>APAEILNGKEISAQIRARLKNQVTQLKEQVPGFTPRLAILQVGNRDDSNLYINVKLKAAEEIGIKATHIKLPRTTTESEVMKYITSLNEDSTVHGFLVQLPLDSENSINTEEVINAIAPEKDVDGLTSINAGRLARGDLNDCFIPCTPKGCLELIKETGVPIAGRHAVVVGRSKIVGAPMHDLLLWNNATVTTCHSKTAHLDEEVNKGDILVVATGQPEMVKGEWIKPGAIVIDCGINYVPDDKKPNGRKVVGDVAYDEAKERASFITPVPGGVGPMTVAMLMQSTVESAKRFLEKFKPGLEHHHHHH[4x]

Methylenetetrahydrofolate dehydrogenase/cyclohydrolase 2 (MTHFD2) is a bifunctional metabolic enzyme found in mitochondria, exhibiting both dehydrogenase and cyclohydrolase catalytic activities. In one-carbon metabolism, MTHFD2 converts 5, 10-methylene tetrahydrofolate (5,10-CH2-THF) to 10-formyl tetrahydrofolate (10-CHO-THF) in mitochondria, thereby regulating the production of NADH, purines, and pyrimidines. An isozyme, methylenetetrahydrofolate dehydrogenase, cyclohydrolase and formyltetrahydrofolate synthetase 1 (MTHFD1), performs similar catalytic reactions to MTHFD2, albeit localized in the cytoplasm rather than the mitochondrion. The key distinction between these two proteins lie in their expression profiles: MTHFD1 is typically expressed in normal cells while MTHFD2 is abundantly expressed in immortal, embryonic, and cancer cells, but absent in adult normal cells.

LY374571 was a competitive inhibitor of human MTHFD1 (IC50 = 630 nM) and MTHFD2 (IC50 = 80 nM). To investigate the molecular basis of the selectivity toward MTHFD2 over MTHFD1, cocrystal structures of human MTHFD1 were determined in complex with 16a, 16d, 16e, 16g, and LY374571 in the presence of NADP+, with resolutions ranging from 1.99 to 2.50 Å. Superimposition of the MTHFD1/16e complex structure with MTHFD1/LY374571 complex structure uncovered several differences between them. First, in the structure of MTHFD1/LY374571, the nicotinamide group of NADP+ was hydrogen bonded with the NH2 moiety of the triaminopyrimidine headgroup of LY374571. However, the addition of a chloride substituent on the phenyl ring in 16e induced a clash with the nicotinamide group of NADP+, leading to the shift of the nicotinamide group of NADP+ away from the triaminopyrimidine headgroup of 16e and the consequent loss of the hydrogen bond between 16e and NADP+ Instead, NADP+ in MTHFD1/16e structure was found to be hydrogen bonded with the side chain of Thr279. Second, in comparison with the MTHFD1/LY374571 structure, it was observed that the addition of the chloride atom in 16e led to the rotation of the phenyl ring by approximately 26°, accompanied by the movement of the γ-carboxylic acid away from β strand h1. The shift of γ-carboxylic acid in 16e resulted in the loss of the van der Waals interactions with Leu51, Tyr52 and Tyr240. These effects collectively contributed to the weaker inhibitory activity of 16e toward MTHFD1 and consequently improved its selectivity to MTHFD2, as shown by the increase in the selectivity index from 7.9 to 27.1 compared with LY374571.> SMSSFEGQMAEYPTISIDRFDRENLRARAYFLSHCHKAHMKGLRAPTLKRRLECSLKVYLYCSPVTKELLLTSPKYRFWKKRIISIEIETPTQISLVDEASGEKEEIVVTLLPAGHCPGSVMFLFQGNNGTVLYTGDFRLAQGEAARMELLHSGGRVKDIQSVYLDTTFCDPRFYQIPSREECLSGVLELVRSWITRSPYHVVWLNCKAAYGYEYLFTNLSEELGVQVHVNKLDMFRNMPEILHHLTTDRNTQIHACRHPKAEEYFQWSKLPCGITSRNRIPLHIISIKPSTMWFGERSRKTNVIVRTGESSYRACFSFHSSYSEIKDFLSYLCPVNAYPNVIPVGTTMDKVVEILKPLCRS

Artemis (SNM1C/DCLRE1C) is an endonuclease that plays a key role in development of B- and T-lymphocytes and in dsDNA break repair by non-homologous end-joining (NHEJ). Artemis is phosphorylated by DNA-PKcs and acts to open DNA hairpin intermediates generated during V(D)J and class-switch recombination. Artemis belongs to a superfamily of nucleases containing metallo-β-lactamase (MBL) and β-CASP (CPSF-Artemis-SNM1-Pso2) domains. The overall fold of the catalytic core of Artemis is similar to that of SNM1A and SNM1B (2 Å backbone RMSD); it has all the key structural characteristics of human MBL fold nucleases, with the di-metal containing active site at the interface between the MBL and β-CASP domains.

We crystallized three forms of truncated Artemis (aa 1–361) with substitutions in several of these metal ion co-ordinating residues, i.e. D37A, H33A, and the Omenn Syndrome patient mutation H35D. The overall architecture of the three variants is almost identical to WT Artemis. The D37A structure crystallizes with only one nickel ion (M1); Both the H33A and H35D variants exhibited loss of the M1 ion. By contrast, all three variants retained the Zn ion in the zinc finger-like motif of the β-CASP domain. Mutation of Asp37 to alanine results in the loss of the second metal in the catalytic site, likely explaining the loss of activity, although the first metal ion is still present. By contrast the D37A variant has similar thermal stability as the WT Artemis, suggesting that it is folded in the presence of a single metal ion in the active site. Our D37A, H33A, and H35D variants lost the ability to digest DNA substrate in vitro, in accord with results with full-length variants. Thus, whilst our results support the importance of having both metals for the nuclease activity by Artemis, subtle features can influence MBL fold enzyme activity.> LLSALEDLEVLSRELIEMLAISRNQKLLQLEEENQVLELLIHRDGDFQELMKLALNQGKVHHEMQALEKEVEKRDSDIQQLQKQLKEAEQILATAVYQAK;> MAAVDIRDNLLGISWVDSSWIPILNSGSVLDYFSERSNPFYDRTCNNEVVKMQRLTLEHLNQMVGIEYILLHAQEPILFIIRKQQRQSPAQVIPLADYYIIAGVIYQAPDLGSVINSRVL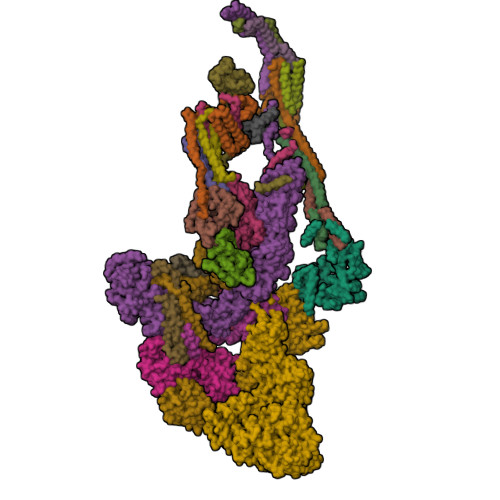TAVHGIQSAFDEAMSYCRYHPSKGYWWHFKDHEEQEKVKPKAKRKEEPSSIFQRQRVDALLIDLRQKFPPRFVQQKSGEKPVPVDQAKKEAEPLPETVKSEEKESTKNIQQTVSTKGPPEKRMRLQ;> PPPPMQYIKEYTDENIQEGLAPKPPPPIKDSYMMFGNQFQCDDLIIRPLESQGIERLHPMQFDHKKELRKLNMSILINFLDLLDILIRSPGSIKREEKLEDLKLLFVHVHHLINEYRPHQARETLRVMMEVQKRQRLETAERFQKHLERVIEMIQNC;> QLEASLDALLNQVADLKNSLGSFIYKLENEYDRLTWPSVLDSFALLSGQLNTLNKVLKHEKTPLFRNQVIIPLVLSPDRDEDLMRQTEGRVPVFSHEVVPDHLRTKPDPEVEEQEKQLTTDAARIGADAAQKQIQSLNKMCSNLLEKISKEERESESGGLRPNKQTFNPGDTNALVAAVA;> FLPLVHNVIKCMDKDSPDLHQDLNALKTKFQELRKLIGTMPGIHVSPEQQQQQLHSLREQVRTKNELLQKYKSLCM;> NERLRALEDIEREIGAILQNAGTAILELSKEKTNERLLDRQAAAFTTSVQHVEAELSAQIRYLTQVATGQPHEGSSYSSRKDCQMALKRVDYARLKISDVARTCEQML;> MAPVQLDNHQLIPPGGGGGSSGGGGSSSGSASAPAPPPPAAAVAAAAAAAASPGYRLSTLIEFLLHRAYSELMVLTDLLPRKSDVERKIEIVQFASRTRQLFVRLLALVKWANDAGKVEKCAMISSFLDQQAILFVDTADRLASLARDALVHARLPSFAIPYAIDVLTTGSYPRLPTCIRDKIIPPDPITKIEKQATLHQLNQILRHRLVTTDLPPQLANLTVANGRVKFRVEGEFEATLTVMGDDPEVPWRLLKLEILVEDKETGDGRALVHSMQIDFIHQLVQSRLFADEKPLQDMYNCLHCFCLSLQLEVLHSQTLMLIRERWGDLVQVERYHAGKSLSLSVWNQQVLGRKTGTASVHKVTIKIDENDVSKPLQIFHDPPLPASDSKLVERAMKIDHLSIEKLLIDSVHARAHQRLQELKAILRSFNANESSSIETALPALIVPILEPCGNSECLHIFVDLHSGMFQLMLYGLDPATLEDMEKSLNDDMKRIIPWIQQLKFWLGQQRCKQSIKHLPTITTETLQLANYSTHPIGSLSKNKLFIKLTRLPQYYIVVEMLEVPNKPTQLSYNYYFMSVSTADREDSPVMALLLQQFKDNIQDLMSYTKTGKQTRTGTKHKLSDDPCPIDSKKAKRSGEMCAFNKVLAHFVAMCDTNMPFVGLRLELSNLEIPHQGVQVEGDGFNHAIRLLKIPPCKGISEETQKALDRSLLDCTFRLQGRNNRTWVAELVFANCPLNGTSTREQGPSRHVYLTYENLLSEPVGGRKVVEMFLNDWSSIARLYECVLEFARSLPEIPAHLNIFSEVRVYNYRKLILCYGTTKGSSISIQWNSIHQKFHIALGTVGPNSGCSNCHNTILHQLQEMFNKTPNVVQLLQVLFDTQAPLNAINKLPTVPMLGLTQRTNTAYQCFSILPQSSTHIRLAFRNMYCIDIYCRSRGVVAIRDGAYSLFDNSKLVEGFYPAPGLKTFLNMFVDSNQDARRRSVNEDDNPPSPIGGDMMDSLISQLQPPQQQPFPKQPGTSGAYPLTSPPTSYHSTVNQSPSMMHTQSPGNLHAASSPSGALRAPSPASFVPTPPPSSHGISIGPGASFASPHGTLDPSSPYTMVSPSGRAGNWPGSPQVSGPSPATRLPGMSPANPSLHSPVPDVSHSPRAGTSSQTMPTNMPPPRKLPQRSWAASIPTILTHSALNILLLPSPTPGLVPGLAGSYLCSPLERFLGSVIMRRHLQRIIQQETLQLINSNEPGVIMFKTDALKCRVALSPKTNQTLQLKVTPENAGQWKPDELQVLEKFFETRVAGPPFKANTLIAFTKLLGAPTHILRDCVHIMKLELFPDQATQLKWNVQFCLTIPPSAPPIAPPGTPAVVLKSKMLFFLQLTQKTSVPPQEPVSIIVPIIYDMASGTTQQADIPRQQNSSVAAPMMVSNILKRFAEMNPPRQGECTIFAAVRDLMANLTLPPGGRPXXXXXXXXXXXXXXXXXXXXXXXXXXXXXXXXXXXXXXXXXXXXXXXXXXXXXXXXXXXXXXXXXXXXXXXXXXXXXXXXXXXXXXXXX;> QPLLDAVLANIRSPVFNHSLYRTFVPAMMAIHGPPIVSPVVCSRKRRFEEDERQSIPNVLQGEVARLDPKFLVNLDPSHCSNNGTVHLICKLDDKDLPSVPPLELSVPADYPAQSPMWIDRQWQYDANPFLQSVHRCMTSRLLQLPDKHSVTALLNTWAQSIHQACL;> MDLAYVCEWEKWAKSTYCPSLPLACAWSCRNLIAFTTDLRNDDQDLTHMIHILDTEHPWEVHSVSSGHSEAITCLEWDQSGSRLLSADADGQIKCWSMADHLANSWESSVGSQVEGDPIVALSWLHNGVKLALHVEKSGASSFGEKFSRVKFSPSLTLFGGKPMEGWIAVTVSGLVTVSLLKPSGQVLTSTESLCRLRGRVALADIAFTGGGNIVVAAADGSSASPVKFYKVCVSVVSEKCRIDTEILPSLFMRCTTDPNRKDRFPAITHLKFLARDMSEQVLLCASSQTSSLVECWSLRKEGLPVNNIFQQISPVVGDKQPMILKWRILSATNDLDRVSAVALPKLPISLTNTDLKVASDTQFYPGLGLALAFQDGSVHMVHRLSLQTMAVFYSSAPRSLDEPALKRPRTTCPAVHFKAMQLSWTSLALVGIDNHGKLSMLRISPSLGHPLEPKLALQHLLFLLEYCMVTGYDWWDILLHVQPGMVQSLVERLHEEYTRQKPALQQVLSTRILAMKASLCKLSPCTVARVCDYHTKLFLMAITSTLKSLLRPHFLNTPDKSPGDRLAEICAKITDVDIDKVMINLKTEEFVLDMNTLQALQQLLQWVGDFVLYLLVSLPNQGSPLRPGHSFLRDGTSLGMLRELMVVIRIWGLLKPSCLPVYTATSDTQDSMSLLFRLLTKLWICCRDEGAASEPDEGLVDECCLLPSQLLVPNLDWLPASDGLVSRLQPKQPLRLRFGRAPTLPSSTSTLQLDGLTRAPGQPKIDHLRRLHLGAYPTEECKACTRCGCVTMLKSPNKTTAVTQWEQRWIKNCLCGGLWRRVPLSCS;> CEKQVQEVGLDGTETYLQPLSMSQNLARLAQRIDFSQGSGSEEEEAAGPDGDAPDWGGAGADQDDEEGLVKFQPSLWPWDSVRNNLRSALTEMCVLYDVLSIVRDKKFMTLDPVSQDALPPKQSPQTLQLISKKKSLAGAAQILLKGAERLTKSVAENQENKLQRDFNSELLRLRQHWKLRKVGDKILGDLSYRSAGSLFPHHGTFEVIKNTDIDLDKKIPEDYCPLDVQIPSDLEGSAYIKVSIQKQAPDIGDLGTVNLFKRPLPKSKPGSPHWQTKLEAAQNVLLCKEIFAQLSREAVQIKSQIPHIVVKNQIISQPFPSLQLSISLCHSSDDKKSQKCAAEKPGQEDHLYVLEHNLHLLIREFHKQTLSSIVMPHPASAPFGHKRMRLSGPQAFDKNEINSIQSTEGLLEKIIKQAKHIFLRSRTAATIDSLASRIEDPQIQAHWSNINDVYESSVKVLITSQGYEQICKSIQLQLNIGVEQVRVVHRDGRVIMLSHQEQELQDFLLSQMSQHQVHAVQQLAKVMGWQVLSFSNHVGLGPIESIGNASAITVASPSGDYAISVRNGPESGSKIMVQFPRNQCKDLPKSDVLQDSKWSHLRGPFKEVQWNKMEGRNFVYKMELLMSALS;> NMMEYLLQGSVLDHSLESLIHRLRGLCDNMEPETFLDHEMVFLLKGQQASPFVLRARRSMDRAGAPWHLRYLGQPEMGDKNRHALVRNCVDIATSENLTDFLMEMGFRMDHEFVAKGHLFRKGIMKVVVYKIFRILVPGNTDSTEALSLSYLVELSVVAPAGQDMVSDDMRNFAEQLKPLVHLEKID;> VTCVSQMPVAEGKSLQQTVELLTKKLEMLGAEKQGTFCVDCETYHTAASTLGSQGQAGKLMYVMHNSEYPLSCFALFENGPCLIADTNFDVLMVKLKGFFQSAKASKIETRGTRYQYCDFLVKVGTVTMGPSARGISVEVEYGPCVVASDCWSLLLEFLQSFLGSHAPGAPTVFGNRHDAVYGPADTMIQYMELFNKI;> DRLTQLQDAVNSLADQFCNAIGVLQQCGPPASFSNIQTAINKDQPANPTEEYAQLFAALIARTAKDIDVLIDSLPSEESTAALQAASLYKLEEENHEAATCLEDVVYRGDMLLEKIQSALADIAQS;> QSKETLLQSYNKRLKDDIKSIMDNFTEIIKTAKIEDETQVSRATQGEQDNYEMHVRAANIVRAGESLMKLVSDLKQFLILNDFPSVNEAIDQRNQQLRALQEECDRKLITLRDEVSIDLYELEEEYYSSSS;> METQLQSIFEEVVKTEIIEEAFPGMFMDTPEDEKTKLISCLAAFRQFWSGLSQESHEQCVQWIVKFIHGQHSPKRISFLYDCLAMAVETGLLPPRMVCESLINSDSLEWERTQLWALTFKLVRKIIGGVDYKGVRDLLKAILEKILTIPNTVSSAVVQQLLAAREVIAYILERNACLLPAYFAVTEIRKLYPEGKLPHWLLGNLVSDFVDTFRPTARINSICGRCSLLPVVNNSGAICNSWKLDPATLRFPLKGLLPYDKDLFEPQTALLRYVLEQPYSRDMVCNMLGLNKQHKQRCPVLEDQLVDLVVYAMERSETEEKFDDGGTSQLLWQHLSSQLIFFVLFQFASFPHMVLSLHQKLAGRGLIKGRDHLMWVLLQFISGSIQKNALADFLPVMKLFDLLYPEKECIPVPDINKPQSTHAFAMTCIWIHLNRKAQNGDSTLQIPIPHSLKLHHEFLQQSLRNKSLQMNDYKIALLCNAYSTNSECFTLPMGALVETIYGNGIMRVPLPGTSCLASASVTPLPMNLLDSLTVHAKMSLIHSIATRVIKLAHTKSSVALAPALVETYSRLLVYMEIESLGIKGFISQLLPTVFKSHAWGILHTLLEMFSHRMHHIQPHYRVQLLSHLHTLAAVAQTNQNQLHLCVESTALRLITALGSSEVQPQFTRFLNDPKTVLSAESEELNRALILTLARATHVTDFFTGSDSIQGTWCKDILQTIMNFTPHNWASHTLSCFPAPLQAFFKQNNVPQESRFNLKKNVEEEYRKWKSMTDENEIITQFSVQGFPPLFLCLLWKMLLETDHISQIGYKVLERIGARALVAHVRTFADFLVYEFSTSAGGQQLNKCIEILNDMVWKYNIVTLDRLILCLAMRSHEGNEAQVCYFIIQLLLLKPNDFRNRVSDFVKENSPEHWLQSDWHTKHMSYHKKYPEKLYFEGLAEQVDPPVPIQSPYLPIYFGNVCLRFLPVFDIVIHRFLELLPVSKSLETLLDHLGGLYKFHDRPVTYLYNTLHYYEMCLRNRDHLKRKLVHAIIGSLKDNRPQGWCLSDTYLKHAMNAREDNPWVPEDSYYCKLIGRLVDTMAGKSPGPFPNCDWRFNEFPNPAAHALHVTCVELMALAVPGKDVGNALLNVVLKSQPLVPRENITAWMNAIGLIITALPEPYWIVLHDRIVNVISSSSLTSETEWVGYPFRLFDFTACHQSYSEMSCSYTLALAHAVWHHSSIGQLSLIPKFLTEALLPVVKTEFQLLYVYHLVGPFLQRFQQERTRCMIEIGVAFYDMLLNVDQCSTHLNYMDPICDFLYHMKYMFTGDSVKEQVEKIICNLKPALKLRLRFITHISKMEPAVPPQALNSGSPAPQSNQVPASLPVTQ;> VNLKQAILQAWKERWSDYQWAINMKKFFPKGATWDILNLAEALLEQAMIGPSPNPLILSYLKYAISSQMVSCSSVLTAISKFDDFSRDLCVQALLDIMDMFCDRLSCHGKAEECIGLCRALLSALHWLLRCTAASAERLQEGLEAGTPAPGEKQLALCLQCLEKTLSSTKNRALLHIAKLEEASSWTAIEHSLLKLGEILANLSNPQLRSQAERCGTLIRSIPSMLSVHSEQLHKTGFPTIHALILLEGTMNLTGEMQPLVEQLMMVKRMQHIPTPLFVLEIWKACFVGLIESPEGTQELKWTAFTYLKIPQVLVKLKKYFHGEKDFTEDVNCAFEFLLKLTPLLDKADQRCNCDCTNFLLQECNKQGLLSEVNFASLVGKRTADRDPQLKSSENANIQPNPGLILRAEPTVTNILKTMDADHSKSPEGLLGVLGHMLSGKSLDLLLAAAAATGKLKSFARKFINLNEFTTHGSGESTKTASVRALLFDISFLMLCHVAQTYGSEVILSESSSGEEVPFFETWMQTCMPEEGKILNPDHPCFRPDSTKVESLVALLNNSSEMKLVQMKWHEACLSISAAILEILNAWENGVLAFESIQKITDNIKGKVCSLAVCAVAWLVAHVRMLGLDEREKSLQMIRQLAGPLYSENTLQFYNERVVIMNSILEHMCADVLQQTATQIKFPSTGVDTMPYWNLLPPKRPIKEVLTDIFAKVLEKGWVDSRSIHILDTLLHMGGVYWFCNNLIKELLKETRKEHTLRAVQLLYSIFCLDMQQVTLVLLGHILPGLLTDSSKWHSLMDPPGTALAKLAVWCALSSYSSHKGQASSRQKKRHREDIEDYVSLFPVEDMQPSKLMRLLSSSDDDANILSSPTDRSMNSSLSASQLHTVNMRDPLNRVLANLFLLISSILGSRTAGPHTQFVQWFMEECVGCLEQDSRGSILQFMPFTTVSELVKVSAMSSPKVVLAITDLSLPLGRQVAAKAIA;> VADVVFVIEGTANLGPYFEELRKHYLLPAIEYFNGGPPAETDFGGDYGGTQYSLVVFNTVDCAPESYVQCHAPTSSAYEFVTWLDGIKFMGGGGESCSLIAEGLSTALQLFDDFKKMREQIGQTHRVCLLICNSPPYLLPAVESTTYSGCTTESLVQKIGERGIHFSIVSPRKLPALRLLFEKAAPPALLEPLQQPADVSQD;> GVNLEAFSQAISAIQALRSSVSRVFDCLKDGMRNKETLEGREKAFIANFQDNLHSVNRDLNELERLSNLVGKPSENHPLHNSGLLSLDPVQDKTPLYSQLLQAYKWSNKLQYHAGLASGLLNQQSLKRSANQMGVSAKRRPKAQPTTLVLPPQYVDDVISRIDRMFPEMSIHLSRPNGTSAMLLVTLGKVLKVIVVMRSLFIDRTIVKGYNESVYTEDGKLDIWSKSSYQVFQKVTDHATTALLHYQLPQMPDVVVRSFMTWLRSYIKLFQAPCQRCGKFLQDGLPPTWRDFRTLEA;> AAPGAPRPSNSTLVDELESSFEACFASLVSQDYVNGTDQEEIRTGVDQCIQKFLDIARQTECFFLQKRLQLSVQKPDQVIKEDVSELRSELQRKDALVQKHLTKLRHWQQVLEDINVQ;> DFDPVQRYKMLIPQLKESLQTLMKVAAQNLIQNTNIDNGQKSSDAPLQRFDKCLEEFYALCDQLELCLRLAHECLSQSCDSAKHSPTLVPTATKPDAVQPDSLPYPQYLAVIKAQITCAKDIHTALLDCANKVT;> EVNTATLCRIGQETVQDIVYRTMEIFQLLRNMQLPNGVTYHTGTYQDRLTKLQDHLRQLSILFRKLRLVYDKCNENCGGMDPIPVEQLIPYVDEDGSKNDDRAGPPRFASEERREIVEVNKKLKQKNQQLKQIMDQLRNLIWDINAMLAMRN;> GNRLRFQLELEFVQCLANPNYLNFLAQRGYFKDKAFVNYLKYLLYWKEPEYAKYLKYPQCLHMLELLQYEHFRKELVNAQCAKFIDEQQILHW7,8-dimethoxy-1,4-dimethylquinolin-2(1H)-one | C13 H15 N O3 | 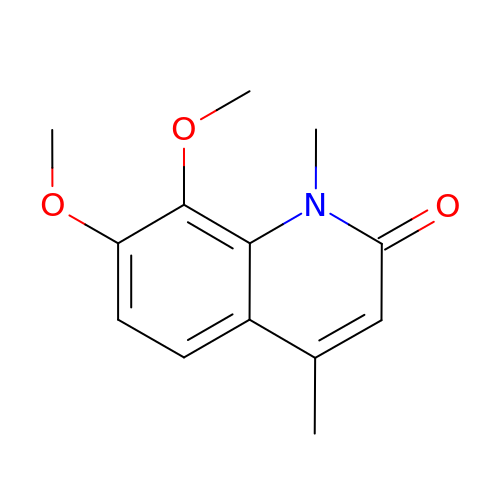DHJBSOKLGMWDBA-UHFFFAOYSA-N> 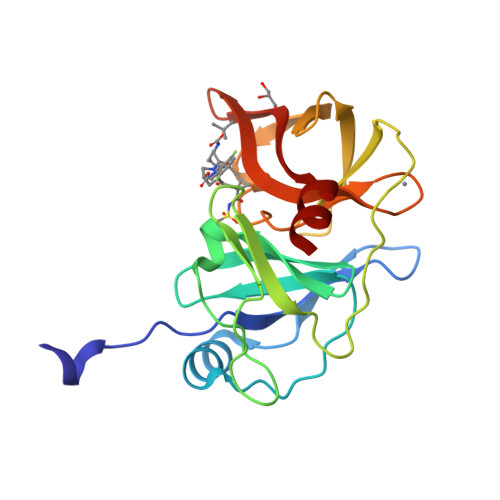HMASMKKKGSVVIVGRINLSGDTAYAQQTRGEEGCQETSQTGRDKNQVEGEVQIVSTATQTFLATSINGVLWTVHHGAGTRTIASPKGPVTQMYTNVDKDLVGWQAPQGSRSLTPCTCGSSDLYLVTRHADVIPVRRRGDSRGSLLSPRPISYLKGSSGGPLLCPAGHAVGIFRAAVSTRGVAKAVDFIPVESLETTM>[3x]XEWEALEKKL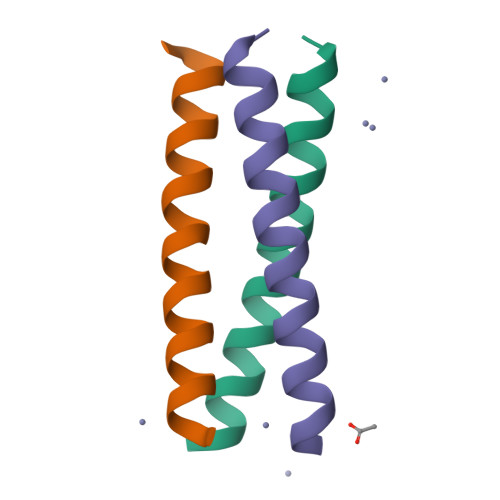AALESKVQALEKKLEALEHGX(1R,9S,12R)-13-[[8-[[1-(2-fluoranyl-2-methyl-propyl)piperidin-4-yl]amino]-3-methyl-[1,2,4]triazolo[4,3-b]pyridazin-6-yl]carbonyl]-12-propan-2-yl-11,13-diazatricyclo[7.3.1.0^{2,7}]trideca-2,4,6-trien-10-one 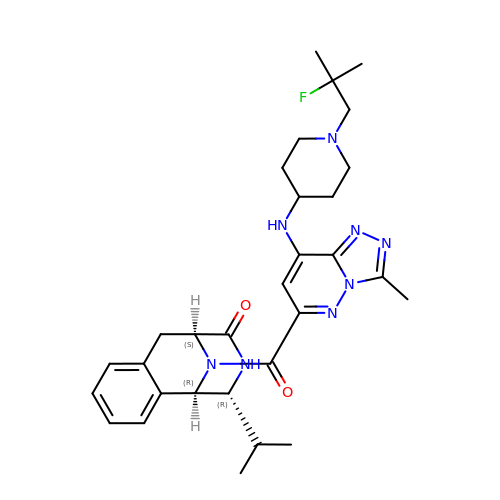| C30 H39 F N8 O2 | NGXAMXNWIHBLBN-JIMJEQGWSA-N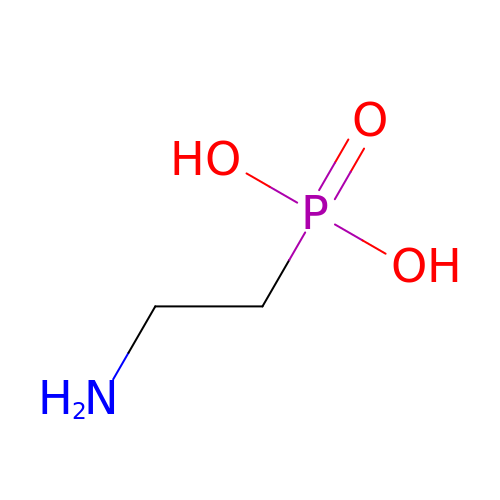(2-aminoethyl)phosphonic acid | C2 H8 N O3 P | QQVDJLLNRSOCEL-UHFFFAOYSA-N1-[3-[5-(7-aminothiazolo[5,4-d]pyrimidin-2-yl)-1-[[(2S)-tetrahydrofuran-2-yl]methyl]imidazol-4-yl]phenyl]-3-(4-methoxyphenyl)urea | C27 H26 N8 O3 S | 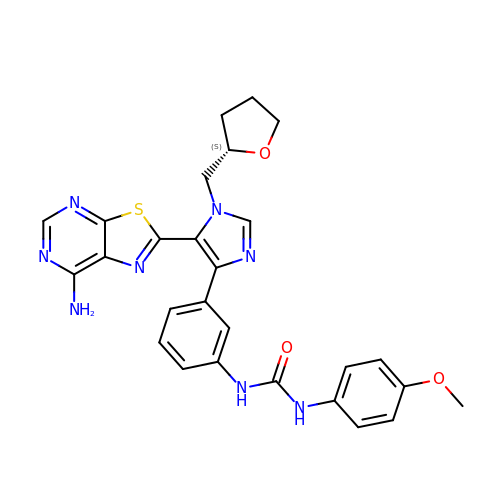ABVBWRLOEHXZBY-FQEVSTJZSA-N>[22x]MAQVINTNSLSLLTQNNLNKSQSALGTAIERLSSGLRINSAKDDAAGQAIANRFTANIKGLTQASRNANDGISIAQTTEGALNEINNNLQRVRELAVQSANSTNSQSDLDSIQAEITQRLNEIDRVSGQTQFNGVKVLAQDNTLTIQVGANDGETIDIDLKQINSQTLGLDSLNVQKAYDVKDTAVTTKAYANNGTTLDVSGLDDAAIKAATGGTNGTASVTGGAVKFDADNNKYFVTIGGFTGADAAKNGDYEVNVATDGTVTLAAGATKTTMPAGATTKTEVQELKDTPAVVSADAKNALIAGGVDATDANGAELVKMSYTDKNGKTIEGGYALKAGDKYYAADYDEATGAIKAKTTSYTAADGTTKTAANQLGGVDGKTEVVTIDGKTYNASKAAGHDFKAQPELAEAAAKTTENPLQKIDAALAQVDALRSDLGAVQNRFNSAITNLGNTVNNLSEVRSRIEDSDYATEVSNMSRAQILQQAGTSVLAQANQVPQNVLSLLR

Salmonella has two flagellin genes, fljB and fliC, and their expression is autonomously regulated to produce either FljB or FliC for filament formation at a frequency of 10−3–10−4 per cell per generation. This is called phase variation, and it is thought to be a mechanism to enable escape from the host immune system by changing flagellar antigenicity. The molecule consists of four domains, D0, D1, D2, and D3, arranged from the inner core to the outer surface of the filament. Domains D0 and D1 form the inner core of the filament and are made of α-helical coiled coils.

We analyzed the structure of the FljB filament by cryoEM single-particle image analysis in one of the two mutant straight forms called the R-type. We used the R-type straight form to utilize the helical symmetry for image analysis as well as to compare the structure with the R-type straight filament formed by FliC. The 3D image of the FljB filament was reconstructed at 3.6 Å resolution from about 1.1 million segment images obtained from 2319 cryoEM movie images. It showed a tubular structure formed by a helical assembly of subunit proteins with an outer diameter of 230 Å and an inner diameter of 20 Å and with a similar helical parameter to the R-type straight filament formed by FliC. The 11 protofilaments could also be recognized as in the FliC filament structure. The missing residues 193–287, corresponding to domain D3, were not built because the resolution of the 3D map was too low to trace the chain. In addition, the density level of domain D3 was much lower than other domains in FljB, indicating that domain D3 was more mobile than other domains of FljB. This indicates that the two-chain hinge connection between domains D2 and D3 was relatively flexible, making domain D3 mobile. When domains D0, D1, and D2 were superimposed between FljB and FliC, domain D3 of FljB was tilted from that of FliC by about 30°, making its position nearly 20 Å higher than that of FliC. Unlike FliC, FljB did not have these contacts, with the corresponding Cα distance between Ala 191 and Thr 350 being 18.4 Å, possibly making the two-chain domain connection less stable and domain D3 oriented differently than FliC.> ECLEIFKACNP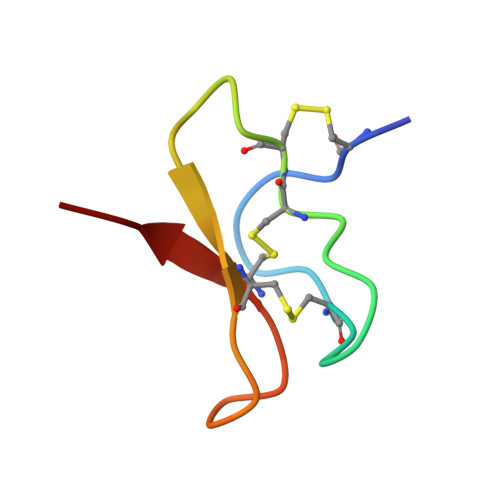SNDQCCKSSKLVCSRKTRWCKYQI> MGHHHHHHGNIT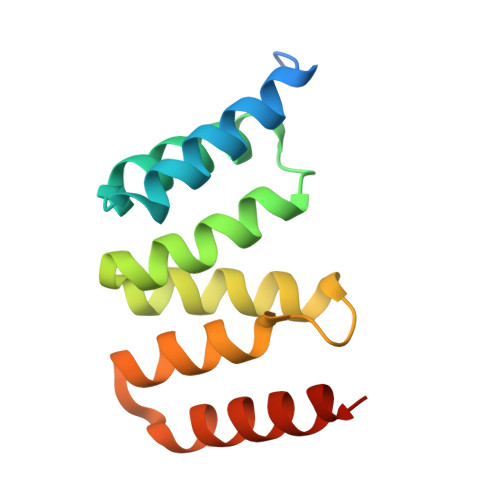LTKRQQEFLLLNGWLQLQCGHAERACILLDALLTLNPEHLAGRRCRLVALLNNNQGERAEKEAQWLISHDPLQAGNWLCLSRAQQLNGDLDKARHAYQHYLELKDHNESP> MASWSHPQFEKGADDDDKVPDPTSVDSVKYSKIKGIPKLDDANDAGGKHSL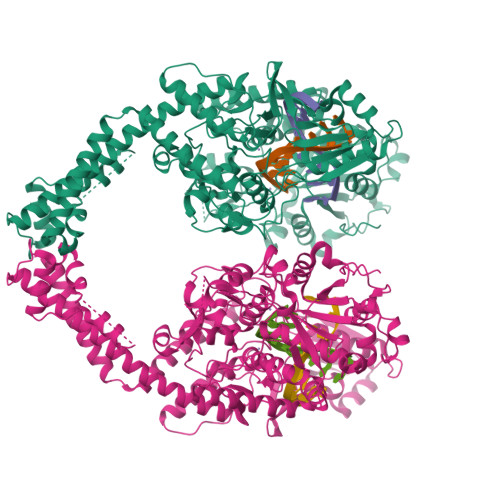ECTLILTEGDSAKSLAVSGLGVIGRDRYGVFPLRGKILNVREASHKQIMENAEINNIIKIVGLQYKKSYDDAESLKTLRYGKIMIMTDQDQDGSHIKGLLINFIHHNWPSLLKHGFLEEFITPIVKASKNKQELSFYSIPEFDEWKKHIENQKAWKIKYYKGLGTSTAKEAKEYFADMERHRILFRYAGPEDDAAITLAFSKKKIDDRKEWLTNFMEDRRQRRLHGLPEQFLYGTATKHLTYNDFINKELILFSNSDNERSIPSLVDGFKPGQRKVLFTCFKRNDKREVKVAQLAGSVAEMSAYHHGEQALMMTIVNLAQNFVGSNNINLLQPIGQFGTRLHGGKDAASPRYIFTMLSTLARLLFPAVDDNLLKFLYDDNQRVEPEWYIPIIPMVLINGAEGIGTGWACKLPNYDAREIVNNVRRMLDGLDPHPMLPNYKNFKGTIQELGQNQYAVSGEIFVVDRNTVEITELPVRTWTQVYKEQVLEPMLNGTDKTPALISDYKEYHTDTTVKFVVKMTEEKLAQAEAAGLHKVFKLQTTLTCNSMVLFDHMGCLKKYETVQDILKEFFDLRLSYYGLRKEWLVGMLGAESTKLNNQARFILEKIQGKITIENRSKKDLIQMLVQRGYESDPVKAWKEAQEKAAEEDETQNQHDDSSSDSGTPSGPDFNYILNMSLWSLTKEKVEELIKQRDAKGREVNDLKRKSPSDLWKEDLAAFVEELDKVESQEREDGAPGFSSISAHHHHHHHHHH>[2x]MEERNHENTLEKDLEAVGQEAQALEERLKAAEEELKGLKDKYLRLLADFDNYRKRMEEELKAREREGVLKALRALLPVLDDLDRALEFA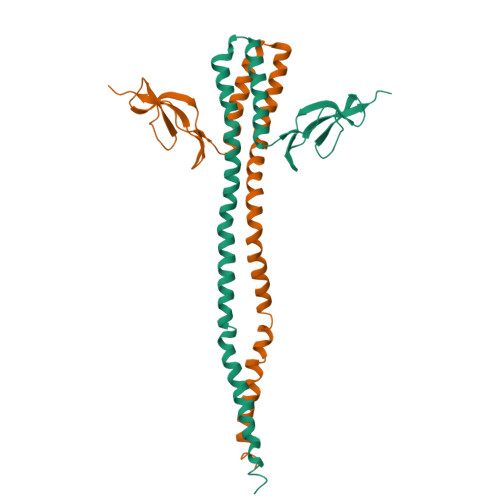EASPESIRQGVRAIRDGFFRILAGLGVEEVPGEGEAFDPRYHEAVGLLPGEPGKVAKVFQRGFRMGEALVRPARVAVGEEKREEADLE> DLKDPIKISIPRYVLCGQGKDAHFEFEVKITVLDETWTVFRRYSRFREMHKTLKLKYAELAALEFPPKKLFGNKD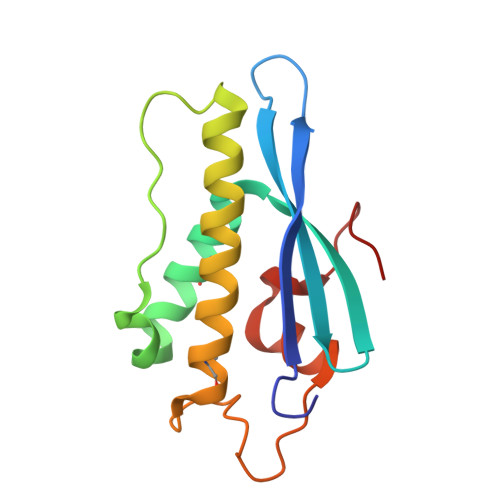ERVIAERRSHLEKYLRDFFSVMLQSATSPLHINKVGLTLSKHTICEFSPFFKKGVFDYS>GSFKFTAQQHVYDINGVKVGGQPGEYPTVLIGSIFYRGHKIVSDGQKGIFDKDAAKALLDQEAELSAETGNPFIIDVLGESVEALTKYVEFILENTTAPFLLDSISPDVRVGALKNLGKDPEIQKRLIYNSIEEHYTEEELAAIKEAGLKTAVILAFSKKALKPNARIDLLQGKDDKEGLIAAAKRAGIEQFLVDPGVLDVASNSWTTEAINVVKEQFGYPGGCAPSAAVYLWKKMRSKGTPFFEVAGAAVFTYPITQGADFILYGPMMNAPWVYRAIATTD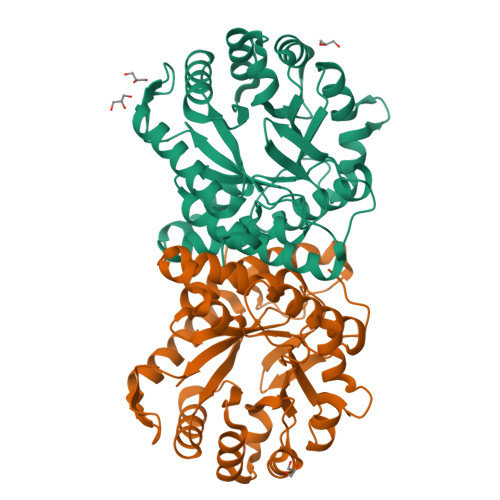AMIAYNNKLTGVKMGTTEHPLLKIF[2x]LAURIC ACID | 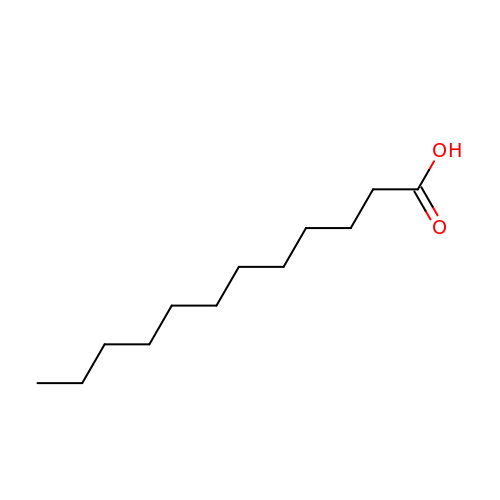C12 H24 O2 | POULHZVOKOAJMA-UHFFFAOYSA-N>MGRIKNKQFAVIGLGRFGGSICKELHRMGHEVLAVDINEEKVNAYASYATHAVIANATEENELLSLGIRNFEYVIVAIGANIQASTLTTLLLKELDIPNIWVKAQNYYHHKVLEKIGADRIIHPEKDMGVKIAQSLSDENVLNYIDLSDEYSIVELLATRKLDSKSIIDLNVRAKYGCTILAIKHHGDICLSPAPEDIIREQDCLVIMGHKKDIKRFENEGM[8x];>[4x]MTLQKDKVIKWVRFTPPQVLAIGFFLTIIIGAVLLMLPISTTKPLSWIDALFTAASATTVTGLAVVDTGTQFTVFGQTVIMGLIQIGGLGFMTFAVLIVMILGKKIGLKERMLVQEALNQPTIGGVIGLVKVLFLFSISIELIAALILSIRLVPQYGWSSGLFASLFHAISAFNNAGFSLWPDNLMSYVGDPTVNLVITFLFITGGIGFTVLFDVMKNRRFKTFSLHTKLMLTGTLMLNAIAMLTVFILEYSNPGTLGHLHIVDKLWASYFQAVTPRTAGFNSLDFGSMREGTIVFTLLLMFIGAGSASTASGIKLTTFIVILTSVIAYLRGKKETVIFRRSIKYPIIIKALAVSVTSLFIVFLGIFALTITEQAPFLQIVFETFSAFGTVGLTMGLTPELTTAGKCIIIVIMFIGRIGPLTFVFSFAKTEQSNIRYPDGEVFTG

The K+ uptake system KtrAB is essential for bacterial survival in low K+ environments. The activity of KtrAB is regulated by nucleotides and Na+. The KtrAB system is composed of the transmembrane KtrB dimer, each containing four structurally similar domains (D1~D4) arranged around a four-fold pseudosymmetry axis normal to the cell membrane, and the regulatory KtrA octamer (tetramer of homodimer) with a ring-like structure, known as the RCK gating ring. ATP binding to KtrA octamer activates K+ flux activity of KtrB, whereas ADP binding inactivates it.

Interestingly, the density at this site was still discernable in Structure II, despite the presence of chelators for divalent ions. The density at the intra-dimer interface of BsKtrA (Structure II) appears to be right on the plane of the horizontal C2 symmetry axis parallel to the membrane, along the BsKtrA dimer interface. Structural refinement of Na+ at the site (Structure II) revealed an octahedral coordination geometry with the distances ranging from 2.50 Å to 2.63 Å, which are within the range of Na+ coordination distance of 2.13 Å to 2.76 Å30. The assigned Na+ is coordinated by the carboxylate oxygens of Glu125 residues and the oxygens in the γ-phosphates of ATPs from both BsKtrA protomers in the intra-dimer interface. The side chains of Arg16 residues reveal an energetically unfavorable conformation pointing to Na+ in the close vicinity. Nevertheless, the repulsive force would be compensated by the γ-phosphates of both ATPs and the carboxylate groups of both Glu125 residues. Second, in the ATP-BsKtrAB structure, the square-shaped ATP-BsKtrA octameric ring causes a steric hindrance for the D1M2b helix of BsKtrB, resulting in a helical hairpin conformation. However, the polar interaction between Arg417 and Thr310 is interrupted in the ATP-BsKtrAB structure, where the side chain of Arg417 forms a hydrogen bond with the exposed carbonyl oxygen of Gly87 located at the kink of the discontinuous D1M2 helix. In ATP-BsKtrAB, the bulky side chain of Phe91 flips away from the pore due to the formation of a helical hairpin. ATP-BsKtrA and BsKtrB mixture in the presence of Na+ revealed a uniform species (black arrow), representing a stable assembly of ATP-BsKtrAB complex as demonstrated by the cryo-EM structure (Structure II) collected from the indicated fraction.> GLGDLIEGVVEGVTRNALTPLTPANNLPDTQSSGPAHSKEIPALTAVETGATNPLVPSDTVQTRHVIQKRTRSESTVESFFARGACVAIIEVDN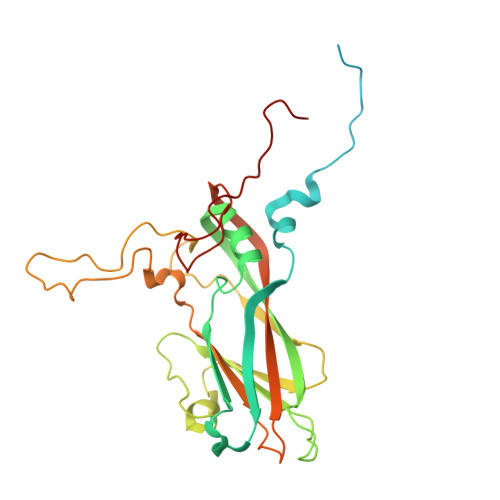DAPTKRASKLFSVWKITYKDTVQLRRKLEFFTYSRFDMELTFVVTSNYTDANNGHALNQVYQIMFIPPGAPIPGKWNDYTWQTSSNPSVFYTYGAPPARISVPYVGIANAYSHFYDGFAKVPLAGQASTEGDSLYGAASLNDFGSLAVRVVNDHNPTKLTSKIRVYMKPKHVRVWCPRPPRAVPYYGPGVDYKDGLAPLPEKGLTTY>[2x]KPPDPPNRVPEKKVVETSAFGHHVQLVNREGKAVGFIEIKESDDEGLDIHISANSLRPGASLGFHIHEKGSCVRPDFES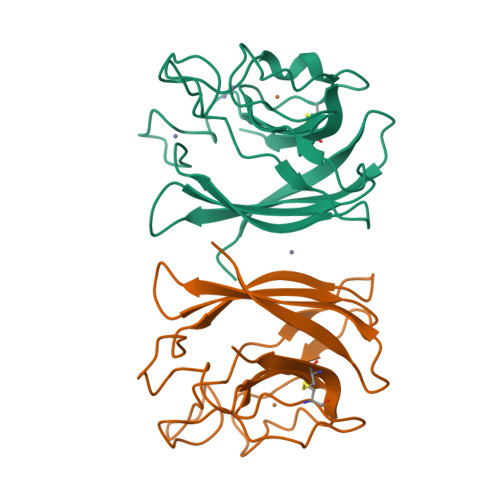AGGHFNPLNKEHGFNNPMGHHAGDLPNLEVGADGKVDVIMNAPDTSLKKGSKLNILDEDGSAFIIHEQADDYLTNPSGNSGARIVCGALLGNNEKQ>MKG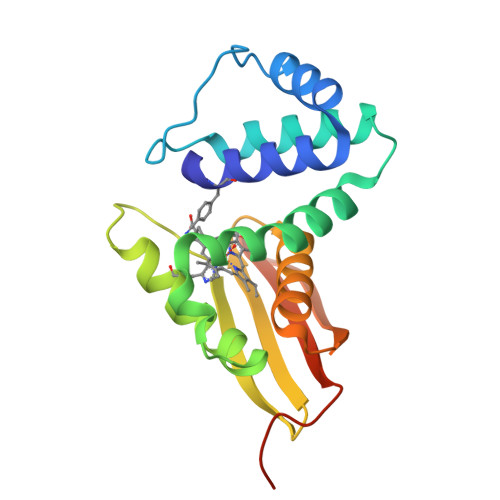TFVGTWIKTLRDLYGNDVVDESLKSVGWEPDRVITPLEDIDDDEVRRIFAKVSEKTGKNVNEIWREVGRQNIKTFSEWFPSYFAGRRLVNFLMMMDEVHLQLTKMIKGATPPRLIAKPVAKDAIEMEYVSKRKMYDYFLGLIEGSSKFFKEEISVEEVERGEKDGFSRLKVRIKFKNPVFEYKKNENLYFQ[2x]4-diazanyl-4-oxidanylidene-butanoic acid | C4 H8 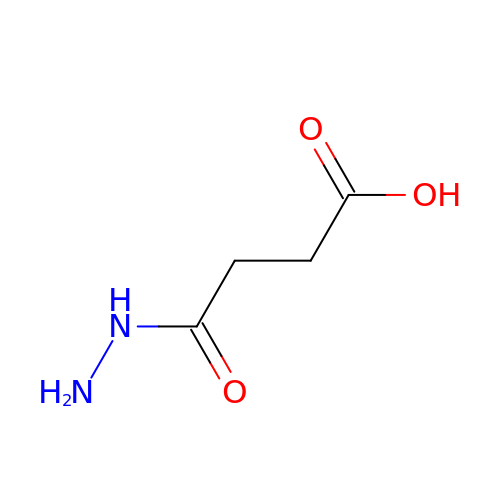N2 O3 | XRMBRQWBOICYRP-UHFFFAOYSA-N> GTAGLGYGSWEIDPKDLTFLKELGTGQFGVVKYGKWRGQYDVAIKMIKEGSMSEDEFIEE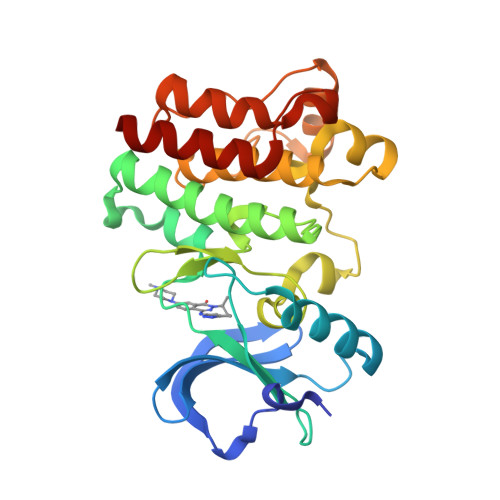AKVMMNLSHEKLVQLYGVCTKQRPIFIITEYMANGCLLNYLREMRHRFQTQQLLEMCKDVCEAMEYLESKQFLHRDLAARNCLVNDQGVVKVSDFGLSRYVLDDEYTSSVGSKFPVRWSPPEVLMYSKFSSKSDIWAFGVLMWEIYSLGKMPYERFTNSETAEHIAQGLRLYRPHLASEKVYTIMYSCWHEKADERPTFKILLSNILDVMDEES> MSKRIALFPALLLALLVIVATALTWMNFSQALPRSQWAQAAWSPNINVIEQMIFHYSLLPRLAISLLVGAGLGLVGVLFQQVLRNPLAEPTTLGVATGAQLGITVTTLWAIPGAMASQFAALAGACVVGLIVFGVAWGKRLSPVTLILAGLVVSLYCGAINQLLVIFHHDQLQSMFLWSTGTLTQTDWGGVERLWPQLLGGVMLTLLLLRPLTLMGLDDGVARNLGLALS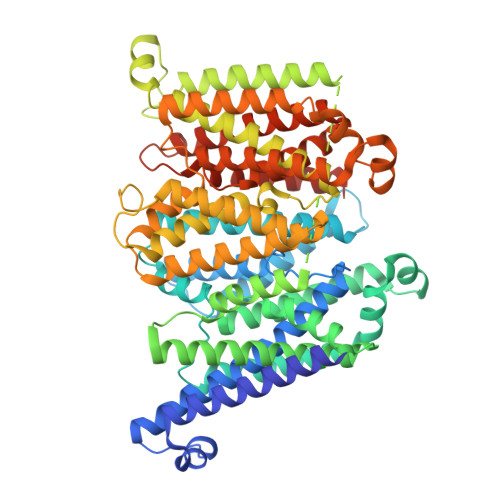LARLAALSLAIVISALLVNAVGIIGFIGLFAPLLAKMLGARRLLPRLMLASLIGALILWLSDQIILWLTRVWMEVSTGSVTALIGAPLLLWLLPRLRSISAPDMKVNDRVATERQHVLAFALAGGVLLLMAVVVALSFGRDAHGWTWASGALLDDLMPWRWPRIMAALFAGVMLAVAGCIIQRLTGNPMASPEVLGISSGAAFGVVLMLFLVPGNAFGWLLPAGSLGAAVTLLIIMIAAGRGGFSPHRMLLAGMALSTAFTMLLMMLQASGDPRMAQVLTWISGSTYNATDAQVWRTGIVMVILLAITPLCRRWLTILPLGGDTARAVGMALTPTRIALLLLAACLTATATMTIGPLSFVGLMAPHIARMMGFRRTMPHIVISALVGGLLLVFADWCGRMVLFPFQIPAGLLSTFIGAPYFIYLLRKQSRHHHHHHHH> QSHLPMPTTPYDTILKAGVVLQLFSHPGAGKTRAIPEYVRQLMTWSNRVYVAGPTRVVAREMLESLQGTKWVCAMVKGLPRPHALARVVVTTHQTLLRYALTSGLLFAKDVSYVLDETHVDSAHTKVLRALIHQTVCKEKSKAACIEMTATGRDSTTGEVRVSMDSNYPIVDRVYNEGVVQAVRKYAETHGPARVAVFVPGLTGKNGALMVAKHIKQTTPYTTIVLSRKTYERNIKLVFKQYPRGMCVVTTSISECGANYDLDAVFDTCQQYHYLVTAVGTKGVITPSTQAQTCQRRGRIGRRREGGYYRPANYDITQAPVLDHPDSVTLLEANMCLRALDLPEEPCGAAVQQAMLRLQPSKDQVYRWLTEQDTETLTEAMAIYSAEGGRRSREQERAIRNRMRSYFNDARWERVEDDAELPAVSPGEYIRDEEGTEVIAGASYVQAPPPYRVRVNQATLLRGSDVKALREEGDRDLAAAIRDEIPEPT

ALSV belongs to the distinct Jingmenvirus group within the Flaviviridae family with segmented RNA genomes. While segments 2 and 4 of the ALSV genome encode the VP1–VP3 proteins of unknown origin, segments 1 and 3 encode the NS2b–NS3 and NS5 proteins, which are related to Flavivirus nonstructural proteins, suggesting an evolutionary link between segmented and unsegmented viruses within the Flaviviridae family. Here, the enzymatic activity of the ALSV NS3-like helicase (NS3-Hel) was characterized and its crystal structure was determined to 2.9 Å resolution. ALSV NS3-Hel exhibits an ATPase activity that is comparable to those measured for Flavivirus NS3 helicases.

D1 and D2 are tandem RecA-like domains with an α/β fold. The proteolytic products were present in the crystals and their proportion was clearly increased in comparison with the sample before crystallization. This result indicates that the missing C-terminal portion of the D3 domain might be owing to proteolytic cleavage that occurred during purification despite the presence of a high concentration of proteinase inhibitor (see Section 2). All conserved SF2 helicase motifs are located in the cleft formed between the D1 and D2 domains. We found that the residues involved in the recognition of NTP, hydrolysis intermediates, catalytic water and metal ion are invariant in ALSV NS3-Hel, which suggests that the catalytic mechanism underlying ATP hydrolysis is conserved in the NS3-Hels from segmented viruses. While most of the catalytic residues of ALSV NS3-Hel superimpose well with their equivalents in ZIKV NS3, the P-loop of ALSV NS3-Hel adopts a different conformation.> HHHNKVRTCWNEGRPALAGWLQLPGTLHAEALARLDYDAVVIDMQHSPIDFGQVAPMLIAIELGGAEPFVRTQVNDPSDIMKLLDAGAYGIIAPMVNTRAEAQTLASALHYSPRGLR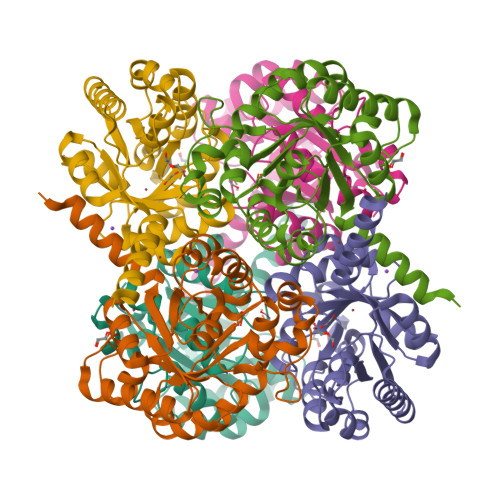SFGPRRPSLRYGSGYLAQASETVVGLAMIETREALANIDEILSVDGIDGVFIGPTDLALDLGHAPLVDTEEAEVVSAIAHVRERAHAAGKRVGIFCGSGGFARVKLAEGFDFVTAAPDLAMLSAAARQVIADARAL> AGGHGDVGMHVKEK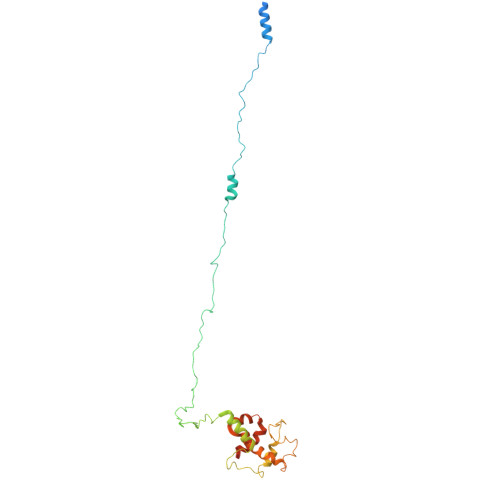EKNKDENKRKDEERNKTQEEHLKEIMKHIVKIEVKGEEAVKKEAAEKLLEKVPSDVLEMYKAIGGKIYIVDGDITKHISLEALSEDKKKIKDIYGKDALLHEHYVYAKEGYCPVLVIQSSEDYVENTEKALNVYYEIGKILSRDILSKINQPYQKFLDVLNTIKNASDSDGQDLLFTNQLKEHPTDFSVEFLEQNSNEVQEVFAKAFAYYIEPQHRDVLQLYAPEAFNYMDKFNEQEINLSLEELKDQR(2R)-hydroxy(phenyl)ethanenitrile 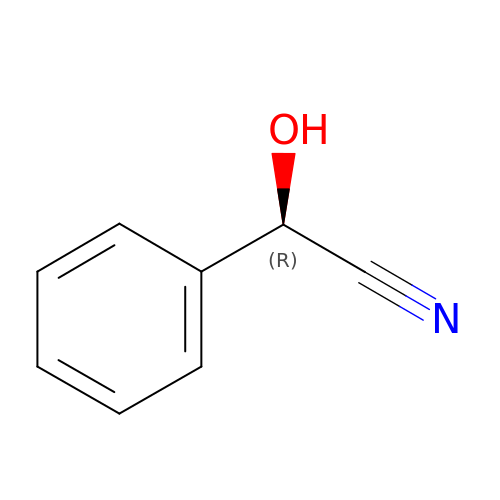| C8 H7 N O | NNICRUQPODTGRU-QMMMGPOBSA-N> EGEDDAEVQQECLHKFSTRDYIM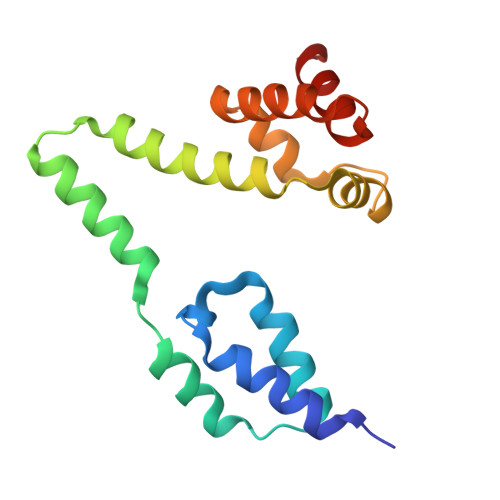EPSIFNTLKRYFQAGGSPENVIQLLSENYTAVAQTVNLLAEWLIQTGVEPVQVQETVENHLKSLLIKHFDPRKADSIFTEEGETPAWLEQMIAHTTWRDLFYKLAEAHPDCLMLNFTVKLISDA> MNTIQQLMMILNSASDQPSENLISYFNNCTVNPKESILKRVKDIGYIFKEKFAKAVGAGCVAIGSQRYKLGVRLYYRVMESMLKSEEERLSIQNFSKLLNDNIFHMSLLACALEVVMATYSRSTSQNLDSGTDLSFPWILNVLNLKAFDFYKVIESFIKAEGNLTREMIKHL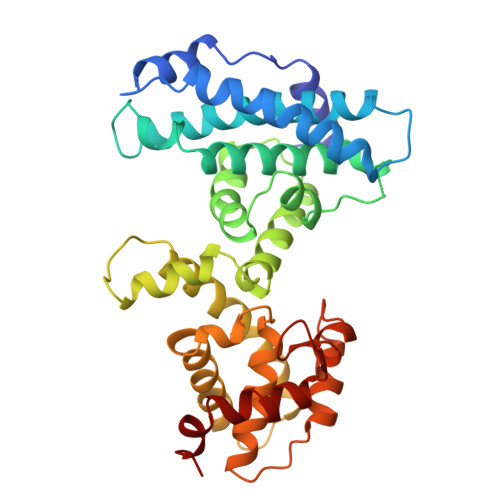ERCEHRIMESLAWLSDSPLFDLIKQSKLVPRGSTSLSLFYKKVYRLAYLRLNTLCERLLSEHPELEHIIWTLFQHTLQNEYELMRDRHLDQIMMCSMYGICKVKNIDLKFKIIVTAYKDLPHAVQETFKRVLIKEEEYDSIIVFYNSVFMQRLKTNILQYA>[12x]RGLASKKTTTVGVIIPDISNIFYAELARGIEDIATMYKYNIILSNSDQNQDKELHLLNNMLGKQVDGIIFMSGNVTEEHVEELKKSPVPVVLAASIESTNQIPSVTIDYEQAAFDAVQSLIDSGHKNIAFVSGTLEEPINHAKKVKGYKRA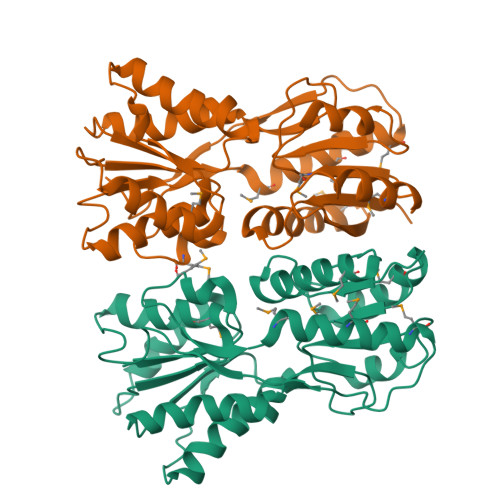LTESGLPVRDSYIVEGDYTYDSGIEAVEKLLEEDEKPTAIFVGTDEMALGVIHGAQDRGLNVPNDLEIIGFDNTRLSTMVRPQLTSVVQPMYDIGAVAMRLLTKYMNKETVDSSIVQLPHRIEFRQSTK>MPLNRTLSMSSLPGLEDWEDEFDLENAVLFEVAWEVANKVGGIYTVLQTKAKVTGDEWGDNYFLVGPYTEQGVRTQVELLEAPTPALKRTLDSMNSKGCKVYFGRWLIEGGPLVVLLDVGASAWALERWKGELWDTCNIGVPWYDREANDAVLFGFLTTWFLGEFLAQSEEKPHVVAHFHEWLAGVGLCLCRARRLPVATIFTTHATLLGRYLCAGAVDFYNNLENFNVDKEAGERQIYHRYCMERAAAHCAHVFTTVSQITAIEAQHLLKRKPDIVTPNGLNVKKFSAMHEFQNLHAQSKARIQEFVRGHFYGHLDFNLDKTLYFFIAGRYEFSNKGADVFLEALARLNYLLRVNGSEQTVVAFFIMPARTNNFNVETLKGQAVRKQLWDTANTVKEKFGRKLYESLLVGSLPDMNKMLDKEDFTMMKRAIFATQRQSFPPVCTHNMLDDSSDPILTTIRRIGLFNSSADRVKVIFHPEFLSSTSPLLPVDYEEFVRGCHLGVFPSYYEPWGYTPAECTVMGIPSISTNLSGFGCFMEEHIADPSAYGIYILDRRFRSLDDSCSQLTSFLYSFCQQSRRQRIIQRNRTERLSDLLDWKYLGRYYMSARHMALSKAFPEHFTYEPNEADAAQGYRYPRPASVPPSPSLSRHSSPHQSEDEEDPRNGPLEEDGERYDEDEEAAKDRRNIRAPEWPRRASCTSSTSGSKRNSVDTA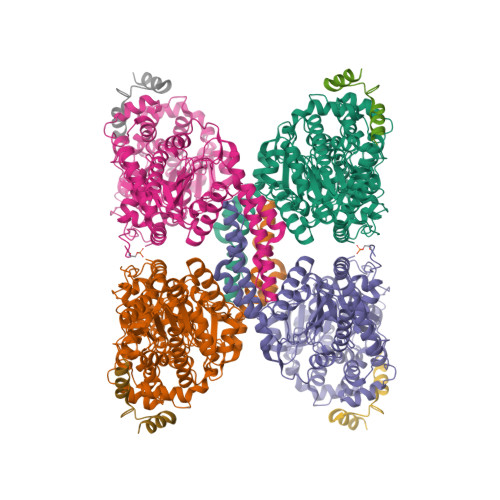TSSSLSTPSEPLSPTSSLGEERN[4x];>[4x]MADQAFVTLTTNDAYAKGALVLGSSLKQHRTTRRLVVLATPQVSDSMRKVLETVFDEVIMVDVLDSGDSAHLTLMKRPELGVTLTKLHCWSLTQYSKCVFMDADTLVLANIDDLFDREELSAAPDPGWPDCFNSGVFVYQPSVETYNQLLHLASEQGSFDGGDQGILNTFFSSWATTDIRKHLPFIYNLSSISIFSYLPAFKVFGASAKVVHFLGRVKPWNYTYDPKTKSVKSEAHDPNMTHPEFLILWWNIFTTNVLPLLQQFGLVKDTCSYVNVEDVSGAISHLSLGEIPAMAQPFVSSEERKERWEQGQADYMGADSFDNIKRKLDTYLQ> VVGGTRAAQGEFPFMVRLSMGCGGALYAQDIVLTAAHCVSGSGNNTSITATGGVVDLQSSSAVKVRSTKVLQAPG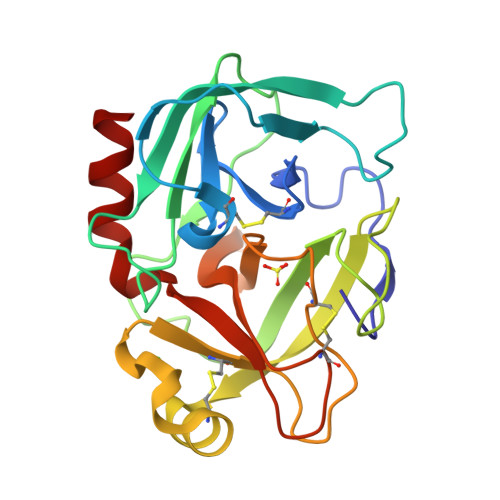YNGTGKDWALIKLAQPINQPTLKIATTTAYNQGTFTVAGWGANREGGSQQRYLLKANVPFVSDAACRSAYGNELVANEEICAGYDTGGVDTCQGDSGGPMFRKDNADEWIQVGIVSWGEGCARKGKYGVYTEVSTFASAIASAARTL>GHMSTTARYDSIGGLFEDFTQSAAQRAIEVRTIFHMIGDVSGKSVLDLACGFGFFGREIYRRGAAKVVGVDISEKMIELAREESRKYGDPLEFHVRDVANMEPLGQFDLVNAAWLFNYADSVENLRKMFKVVRASLKPDGKLVAYTVDPDFSLAKGNFAKYG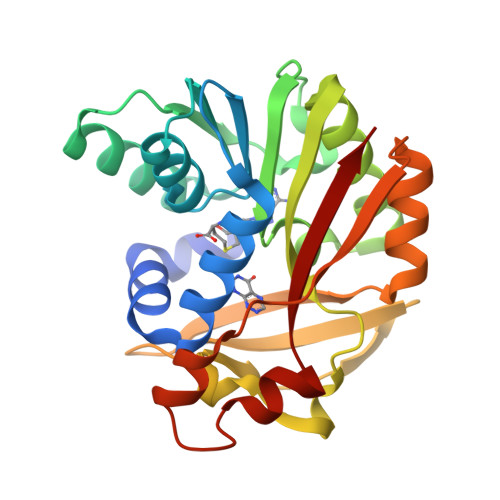VNVLNERAWGPGYRHDAEFVTDPPSQFSFYRWSRADYESAIADAGFSHFEWQKPLLEADDIATHPPGFWDVFQNNCLQTGLVCKP[2x]> ADDIVLKAKNGDVKFP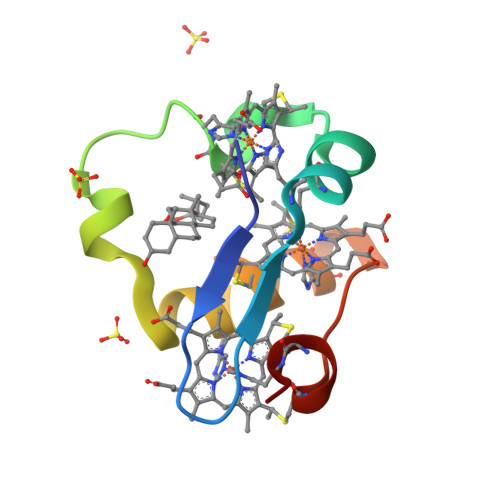HKAHQQAVPDCKKCHEKGPGKIEGFGKEMAHGKGCKGCHEEMKKGPTKCGECHKK> KRRQTSM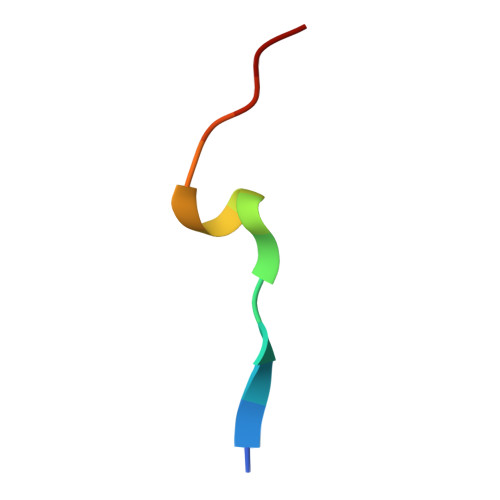TDFYHSKR>[2x]SDLIVKDNALMNASYNLALVEQRLILLAIIEARETGKGINANDPLTVHASSYINQFNVERHTAYQALKDACKDLFARQFSYQEKRERGRINITSRWVSQIGYMDDTATVEIIFAPAVVPLITRLEEQFTQYDIEQ

Typically, BMMFs encode an autonomous plasmid trans-acting replication initiator protein (Rep). Rep binds at an origin of replication on the DNA (termed ori) and in most cases comprises a set of repetitive DNA elements (termed iterons), which are present within most BMMFs. Reps are composed of two winged-helix domains (termed WH1 and WH2) that are essentially a fused N- and C-terminal protein. The Rep described in this study is encoded by the human bioactive bovine meat and milk factor MSBI1.176, which was isolated from a patient with multiple sclerosis.

In this study, we determined the X-ray crystal structure of MSBI1.176 WH1 in the dimeric form to 1.53 Å resolution. The asymmetric unit consisted of one WH1 dimer, i.e. two protomers (termed A and B). However, residues 36–39 could not be fitted into the B protomer owing to a lack of discernible electron density, although the electron density was distinct in the other protomer. The WH1 structure comprised five α-helices (α1–α5) and five β-strands (β1–β5) in each protomer. The A and B protomers were closely related (r.m.s.d. of 0.37 Å); however, a minor structural shift was observed at the β2–β3 hairpin, suggesting some flexibility of this region. Similar to that from RepA, the MSBI1.176 WH1 was also folded as the replication-inert dimer, while RepE (a WH1–2 construct) was crystallized in the monomeric initiator form. Superposition of MSBI1.176 WH1 and RepA WH1 showed that these two domains were structurally similar (r.m.s.d. of 1.20 Å), with both having the typical five α-helices and five β-strands. The MSBI1.176 WH1 hydrophobic pocket also contained three leucine residues, i.e. Leu11, Leu18 and Ile25, which were similarly positioned as in RepA. However, loop movements and different α-helices and β-strands have been observed among the different structures. In the case of MSBI1.176, the β2–β3 hairpin shifted approximately 23 Å when compared with the RepA β2–β3 hairpin. In the MSBI1.176 WH1 structure, six basic residues were also found in this region, i.e. Lys69, Lys73 (both located on α4), Lys85 (β2), Arg90 (β3), Arg78 and Arg96 (both on adjacent loops). The function of the MSBI1.176 WH1 β2–β3 sheet orientation is not obvious, although MSBI1.176 WH1 has a three-amino-acid insertion in the β2 strand that extended the sheet.>[2x]GMVHTKVVIIGSGPAAHTAAIYLSRAELKPVLYEGMLANGTAAGGQLTTTTDIENFPGFPDGIGGAELMENMRKQSIRFGTEVITETI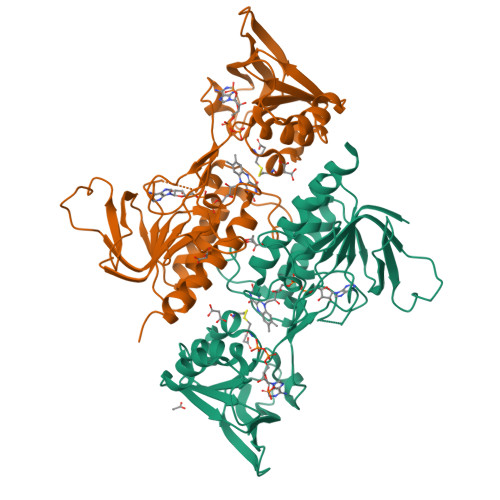SRVDLSSKPFKLWTEWNDGPDKEPACTADAVIIATGANARRLNLPGEETYWQNGISACAVCDGAVPIFRNKPLYVIGGGDSAAEEAMFLAKYGSSVTVLVRRDKLRASKAMAKRLLAHPKVTVRFNTVATEVLGEKKPNGLMTHLRIKNTVTGEEEIVDANGLFYAVGHDPATALVKGQIDLDEDGYIITKPGTSYTSREGVFACGDVQDKRYRQAITSAGSGCIAALEAEKFIAEAESPEEEPVAVSAQKSADNSTIQPAAQEVNGDVKKDPKGAVPEYKSNPLL> GPSQPTYPGDDAPVE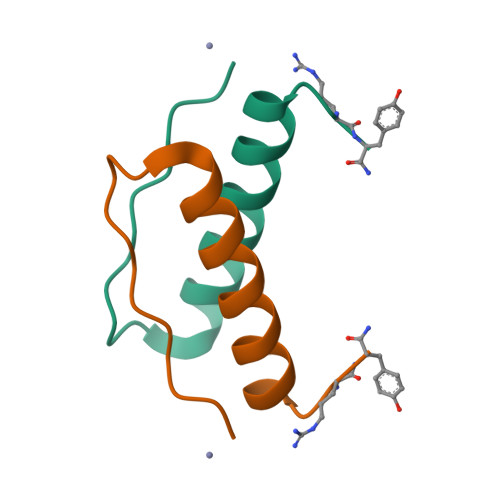DLIRFYNDLQQYLNVVTRHRY N2-({[(4-BROMOPHENYL)METHYL]OXY}CARBONYL)-N1-[(1S)-1-FORMYLPENTYL]-L-LEUCINAMIDE 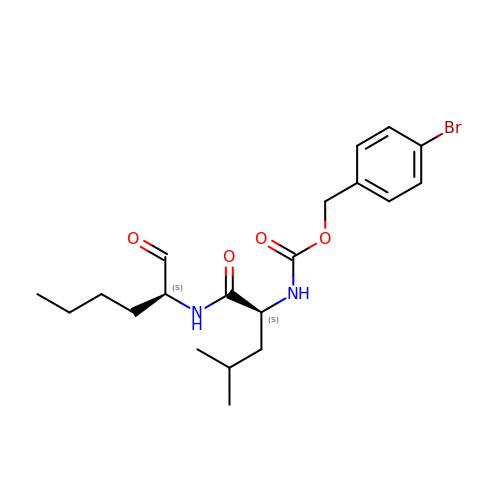| C20 H29 Br N2 O4 | UEDKSAKLZBMNMA-ROUUACIJSA-N Parkinson’s-disease-associated LRRK2 kinase phosphorylates Rab8a and Rab10 to subvert their membrane trafficking functions in the formation of primary cilia. Rab8a is phosphorylated at a threonine (pT72) and subsequently binds to a phosphospecific effector (RILPL2) via its C-terminal RH2 domain. The C-terminal RH2 domain of RILPL2 encodes a Rab-binding domain (RBD) that adopts a parallel α-helical coiled-coil structure. Here, we show that recognition of pT72 involves a dual arginine motif involving R130 and R132 from the RH2 domain of RILPL2.

In addition to complexes, we also determined the structure of uncomplexed Rab8TE. This was performed to support the hypothesis that thermodynamic parameters can be attributed to complex formation rather than intrinsic structural changes from the negative charge at switch 2. The structure of Rab8TE reveals no significant conformational differences in the overall fold relative to the complex Rab8TE:RL2129. Although the structure of uncomplexed pRab8a-pT72 has not yet been determined, it is likely that phosphorylated Rabs do not undergo significant conformational changes upon complex formation with RILPL2.

>GSHMAKTYDYLFKLLLIGDSGVGKTCVLFRFSEDAFNSTFISTIGIDFKIRTIELDGKRIKLQIWDTAGLERFREITTAYYRGAMGIMLVYDITNEKSFDNIRNWIRNIEEHASADVEKMILGNKCDVNDKRQVSKERGEKLALDYGIKFMETSAKANINVENAFFTLARDIKAKMDKKLEGNS[2x]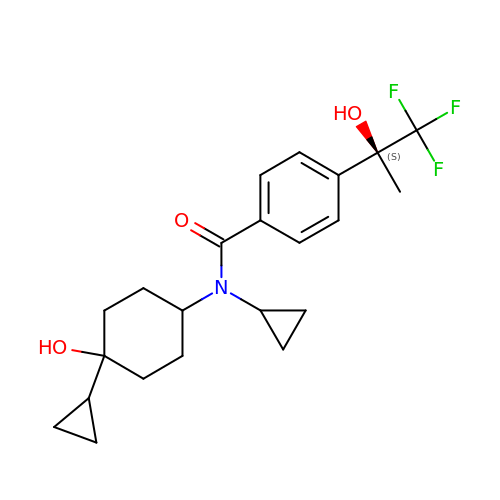N-cyclopropyl-N-(cis-4-cyclopropyl-4-hydroxycyclohexyl)-4-[(1S)-2,2,2-trifluoro-1-hydroxy-1-methylethyl]benzamide | C22 H28 F3 N O3 | SWXZIRVTPISJMP-SESVDKBCSA-N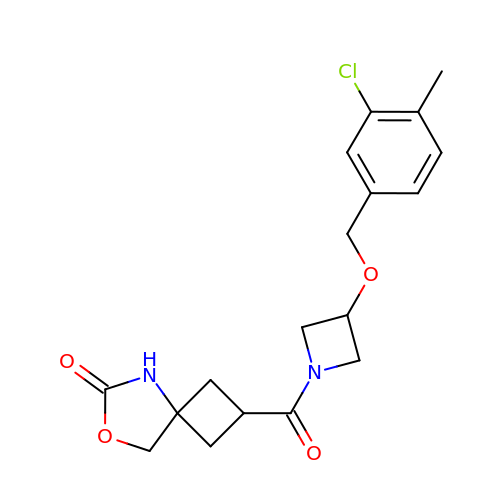(2s,4R)-2-{3-[(3-chloro-4-methylphenyl)methoxy]azetidine-1-carbonyl}-7-oxa-5-azaspiro[3.4]octan-6-one | C18 H21 Cl N2 O4 | AKBHYCHPWZPGAH-QGGXVJLZSA-N> GSIAPYLVKIIDPDYEKNERTRIKAQENLRRIRRKQIAEKGDNEDGTDDPSRRRKIDDLVLNEYENQVALEVVAPEDIPVGFNDIGGLDDIIEELKETIIYPLTMPHLYKHGGALLAAPSGVLLYGPPGCGKTMLAKAVAHESGASFINLHISTLTEKWYGDSNKIVRAVFSLAK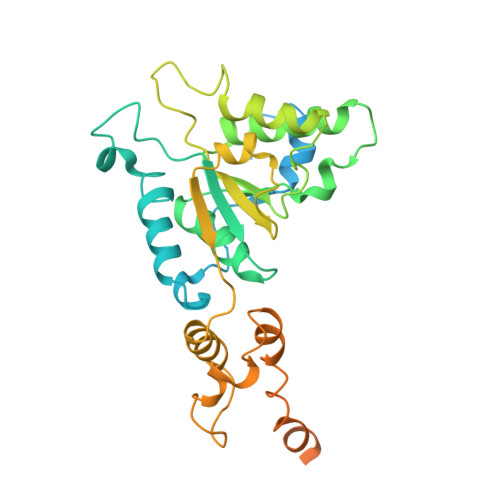KLQPSIIFIDQIDAVLGTRRSGEHEASGMVKAEFMTLWDGLTSTNASGVPNRIVVLGATNRINDIDEAILRRMPKQFPVPLPGLEQRRRILELVLRGTKRDPDFDLDYIARVTAGMSGSDIKETCRDAAMAPMREYIRQHRASGKPLSEINPDDVRGIRTEDFFGRRGGKILSEIPPRQTGYVVQSKNSSEGGYEEVEDDDEQGTAST>[2x]GSMSESADLTELYSIIEKTAQVVDVTASHDKVWPILNAFQDVIADSVISFRASTGSSADDLDCRFTMLPKGLDPYARALEHGLTPKTDHPVGSLLKEVHENLPITSCGVDFGVAGGFTKTWSFPSAEKLGKVSELVKLPSIPDAVAANRDFFEKWGIADMVSTVGIDYSKRTMNLYFGGGVGDRVPAGVFEEKGVRAILGELGLAAPSEELLKFCERSFVIYVTLSWDSPKINRFTYSVMTPEPLGLPVDLAPTFERLIKSAPYDTEGRNYVYGIASTPKGEYHKIASYYQWQKRVEKLLRSDG

The PT EpzP from Streptomyces cinnamonensis DSM 1042 reported here is a member of a new type of bacterial prenyltransferases, as it catalysis the prenylation of a phenazine substrate. EpzP is a soluble, monomeric ABBA PT consisting of 302 amino acids with a molecular mass of 33.2 kDa. The overall structure of EpzP belongs to the PT-fold family and is characterized by ten antiparallel β-strands that assemble into a circular β-barrel. The β-barrel houses a solvent-filled reaction chamber in which the substrates bind and the regioselective Friedel-Crafts prenylation of dhPCA takes place.

Crystallization of unmodified, wild-type EpzP proved initially difficult. However, methylation of the EpzP lysine residues allowed us to grow needle-like crystals (200 mM magnesium chloride, 30% (w/v) PEG4000, Tris hydrochloride pH 8.5) of methylated EpzP (EpzPm). These crystals diffracted to very high resolution of 1.33 Å, belong to the monoclinic space group P21, and were used to assemble a data set for the unliganded protein (EpzPm-nat). Unfortunately, the EpzPm-nat crystals were not suitable for soaking with substrates because the active site is blocked by a symmetry-related protomer from one site, whereas the aromatic binding site is blocked by a PEG molecule. In contrast to EpzPwt, which contains a fully ordered C-terminus that closes the reaction chamber, the structures of EpzPm-SPP and EpzPm-nat have disordered C-termini that cannot be traced beyond residue K292. The lack of an ordered C-terminus renders the aromatic binding site solvent-accessible, and both methylated structures furthermore contain PEG molecules that occupy the cavity. Comparison of EpzPm-nat, which lacks diphosphate or sulfate in the binding pocket, with EpzPwt and EpzPm-SPP revealed different side chain conformations of W119. In the unbound state, the side chain of W119 is rotated by 180°. Furthermore, residues R62 and R49, which both participate in DMAPP binding, adopt alternative conformations when the anion binding site is not fully occupied.3-chloro-5-[2-chloro-5-(1H-indazol-3-ylmethoxy)phenoxy]benzonitrile | C21 H13 Cl2 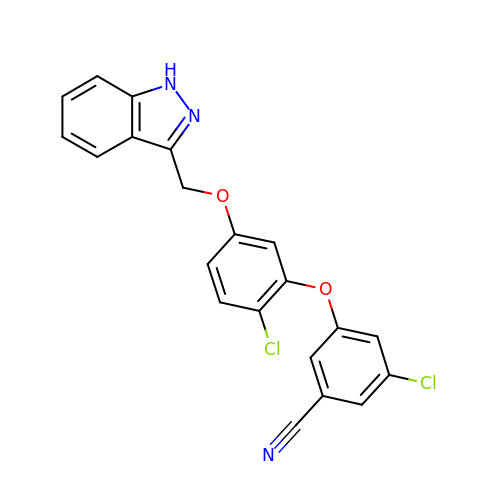N3 O2 | WHCLIFOVZDANCU-UHFFFAOYSA-N>RAITVFSPDGRLFQVEYAREAVKRGATAIGIKCKEGVILIADKRVGSKLLEADTIEKIYKIDEHICAATSGLVADARVLIDRARIEAQINRLTYDEPITVKELAKKICDFKQQYTQYGGVRPFGVSLLIAGVDEVPKLYETDPSGALLEYKATAIGMGRNAVTEFFEKEYRDDLSFDDAMVLGLVAMGLSIESELVPENIEVGYVKVDDRTFKEVSPEELKPYVERANERIRELLKK[7x];>TTTVGLVCKDGVVMATEKRATMGNFIASKAAKKIYQIADRMAMTTAGSVGDAQFLARIIKIEANLYEIRRERKPTVRAIATLTSNLLNSYRYFPYLVQLLIGGIDSEGKSIYSIDPIGGAIEEKDIVATGSGSLTAYGVLEDRFTPEIGVDEAVELAVRAIY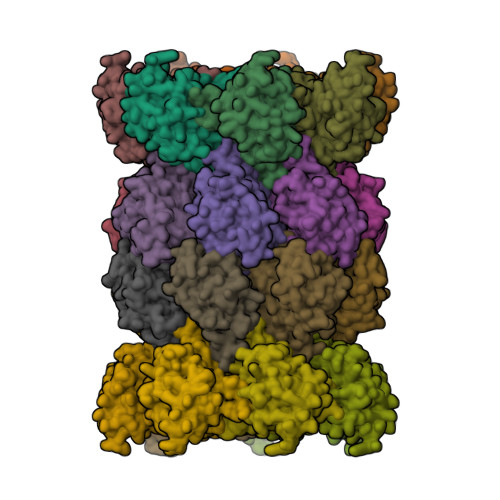SAMKRDSASGDGIDVVKITEDEFYQYSPEEVEQILAKFRK[7x]>[2x]SNAMFSKVNNQKMLEDCFYIRKKVFVEEQGIPEESEIDEYESESIHLIGYDNGQPVATARIRPINETTVKIERVAVMKSHRGQGMGRMLMQAVESLAKDEGFYVATM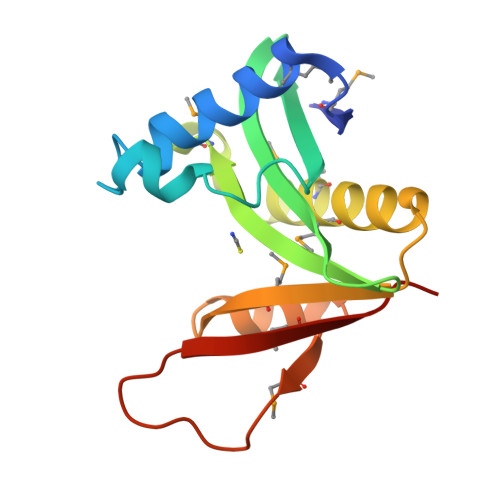NAQCHAIPFYESLNFKMRGNIFLEEGIEHIEMTKKLTSL> MKVHEIPRSQLLKIKQYEGSFVEWYRDLQEDRKKFASLLFRWAAFGYAAREDDGATYISPSQALLERRLLLGDAEDVAIKFLDVLFKGGAPSSSCYSLFYEDFALRDKAKYSGAKREFIEGLATMPLDKIIERIRQDEQLSKIPAEEWLILGAEYSPEEIWEQVAPRIVNVDRSLGKQLRERLGIKCRRPHDAGYCKILMEVVARQLRSHNETYHEYLNQTHEMKTKVANNLTNEFDLVCEFAEVLEEKNYGLGWYVLWQGVKQALKEQKKPTKIQIAVDQLRQPKFAGLLTAKWRALKGAYDTWKLKKRLEKRKAFPYMPNWDNDYQIPVGLTGLGVFTLEVKRTEVVVDLKEHGKLFCSHSHYFGDLTAEKHPSRYHLKFRHKLKLRKRDSRVEPTIGPWIEAALREITIQKKPNGVFYLGLPYALSHGIDNFQIAKRFFSAAKPDKEVINGLPSEMVVGAAALNLSNIVAPVKARIGKGLEGPLHALDYGYGELIDGPKILTPDGPRCGELISLKRDIVEIKSAIKEFKACQREGLTMSEETTTWLSEVESPSDSPRCMIQSRIADTSRRLNSFKYQMNKEGYQDLAEALRLLDAMDSYNSLLESYQRMHLSPGEQSPKEAKFDTKRASFRDLLRRRVAHTIVEYFDDCDIVFFEDLDGPSDSDSRNNALVKLLSPRTLLLYIRQALEKRGIGMVEVAKDGTSQNNPISGHVGWRNKQNKSEIYFYEDKELLVMDADEVGAMNILCRGLNHSVCPYSFVTKAPEKKNDEKKEGDYGKRVKRFLKDRYGSSNVRFLVASMGFVTVTTKRPKDALVGKRLYYHGGELVTHDLHNRMKDEIKYLVEKEVLARRVSLSDSTIKSYKSFAHV

Cas12h1 is a compact CRISPR-associated nuclease from functionally diverse type V CRISPR-Cas effectors and recognizes a purine-rich protospacer adjacent motif (PAM) distinct from that of other type V Cas effectors. Secondly, as a member of subtype V-H, Cas12h1 is distinguished by its relatively small size (870 amino acids), functioning as a compact DNA endonuclease guided by a single crRNA with proficient DNA cleavage capability, highlighting its potential as an efficient genome editing tool. Cas12h1 preferentially nicks the nontarget strand (NTS) of target dsDNA and indiscriminately cleaves ssDNA by collateral cleavage in the RuvC domain. Displaying a “Crab Claw” shape, Cas12h1 contains a distinguishable recognition (REC) lobe and a nuclease (NUC) lobe, with the two lobes connected by the WED domain.

To investigate how Cas12h1 is activated after target recognition, we reconstituted the second ternary complex, which consists of the Cas12h1 D465A mutant, crRNA, and target DNA in the absence of Mg2+; this complex is hereafter referred as the R-loop formation complex (Cas12h1D465A-crRNA-dsDNA). We determined the cryo-EM structure of the Cas12h1 R-loop formation complex at an average resolution of 2.76 Å. Superimposition of the structures shows Cas12h1 undergoes substantial conformational rearrangements from surveillance state to R-loop formation. A comparison of the conformational changes in the lid motif revealed that in the surveillance state, the lid motif was mostly highly flexible (662–670 aa invisible); then, the crRNA:TS heteroduplex helps turn up the lid motif and stabilize the lid in an “open” conformation where the catalytic site is exposed; finally, the NTS turned inwards and was loaded to the catalytic site for cleavage. After target recognition, the lid motif forms new hydrogen bonds with the heteroduplex (S666-A(10), K675-dT(-9), K675-dG(-8)), together with other new hydrogen bonds between D667-Y302, L676-R634, and L660-R680, which stabilize and keep the lid motif in an “open” conformation. The NTS moves ~18 Å towards the catalytic site for first strand cleavage. Moreover, the crRNA and the TS DNA form a 20 bp heteroduplex in the R-loop formation state, in contrast to the 17 bp heteroduplex in the interference state, indicating that the TS has partially disassociated with the crRNA and been loaded into the catalytic site for second strand cleavage.2,6-DICHLOROBIPHENYL | C12 H8 Cl2 | 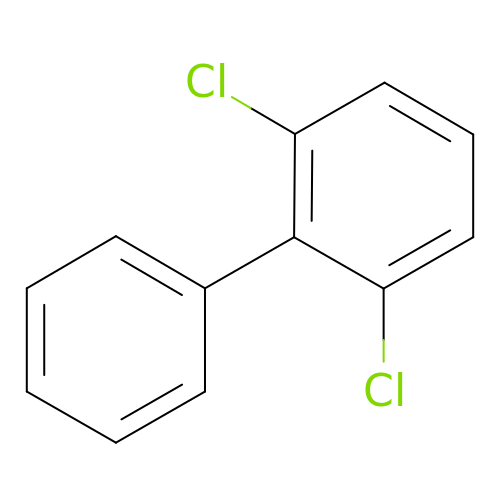IYZWUWBAFUBNCH-UHFFFAOYSA-N2-{4-[2-(2-AMINO-4-HYDROXY-QUINAZOLIN-6-YL)-1-CARBOXY-ETHYL]-BENZOYLAMINO}-PENTANEDIOIC 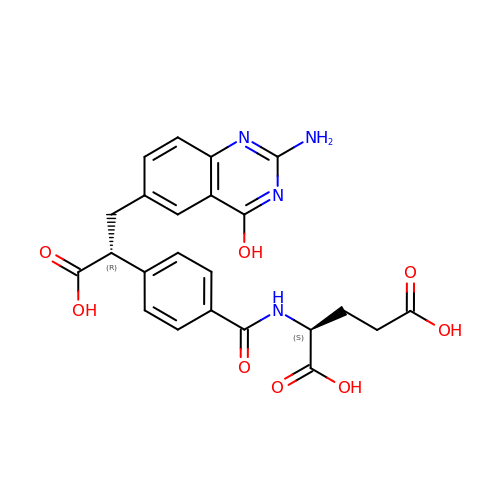ACID | C23 H22 N4 O8 | DAOQLLQRJAXMGY-PBHICJAKSA-N> MSRRAGTPTAKKVTQLVNVEEHVEGFRQVREAHRRELIDDYVELISDLIREVGEARQVDM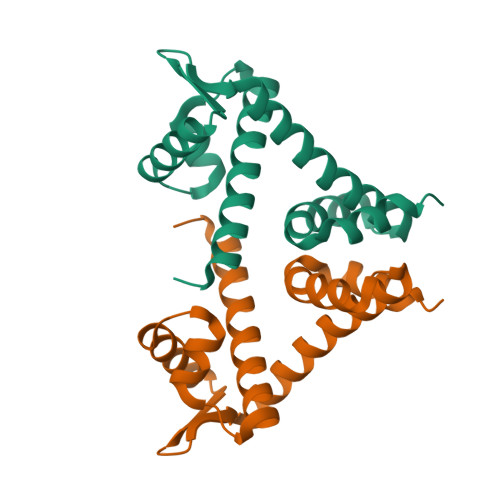AARLGVSQPTVAKMLKRLATMGLIEMIPWRGVFLTAEGEKLAQESRERHQIVENFLLVLGVSPEIARRDAEGMEHHVSEETLDAFRLFTQKHGAK> MASAATGVRAVPGNENSLEIEELARFAVDEHNKKENALLEFVRVVKAKEQIDLTQEWVFTMYYLTLEAKDGGKKKLYEAKVWVKGLT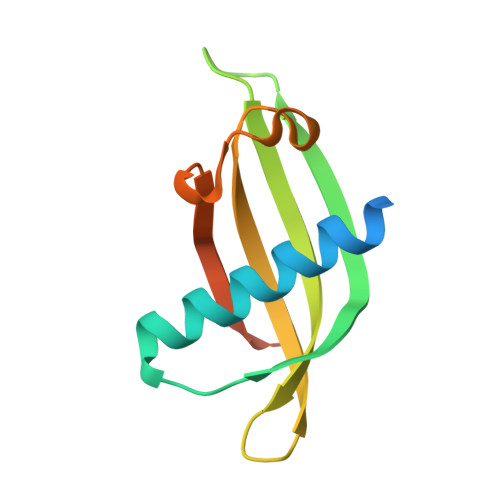NWKLGMNFKELQEFKPVGDAAAAHHHHHH;> MHMEGEYIKLKVIGQDSSEIHFKVKMTTHLKKLKESYCQRQGVPMNSLRFLFEGQRIADNHTPKELGMEEEDVIEVYQEQTGG> GPLGSTNKRKREQISTDNEAKMQIQEEKSP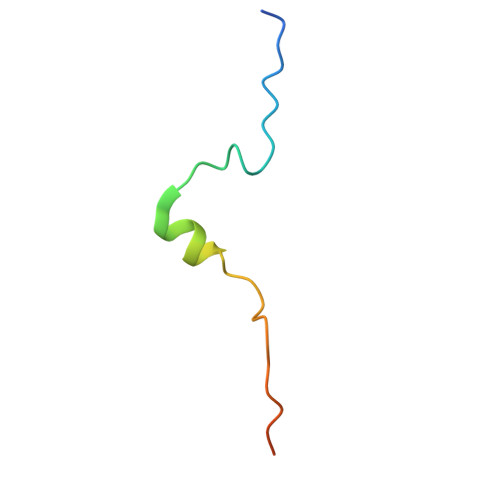KKKRKKRSSKANK>VDSVYRTRSLGVAAEGIPDQYADGEAARVWQLYIGDTRSRTAEYKAWLLGLLRQHGCHRVLDVACGTGVDSIMLVEEGFSVTSVDASDKMLKYALKERWNRRKEPAFDKWVIEEANWLTLDKDVPAGDGFDAVICLGNSFAHLPDSKGDQSEHRLALKNIASMVRPGGLLVIDHKNYDYILSTGCAPPGKNIYYKSDLTKDITTSVLTVNNKAHMVTLDYTVQVPGAGRDGAPGFSKFRLSYYPHCLASFTELVQEAFGGRCQH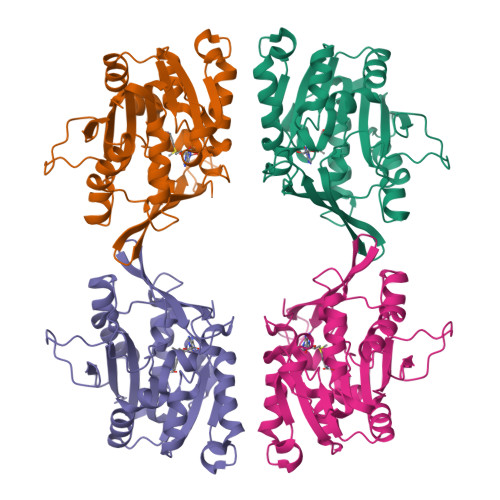SVLGDFKPYRPGQAYVPCYFIHVLKKTG[4x]> SGVDDDMACHKIPVEADFLYAYS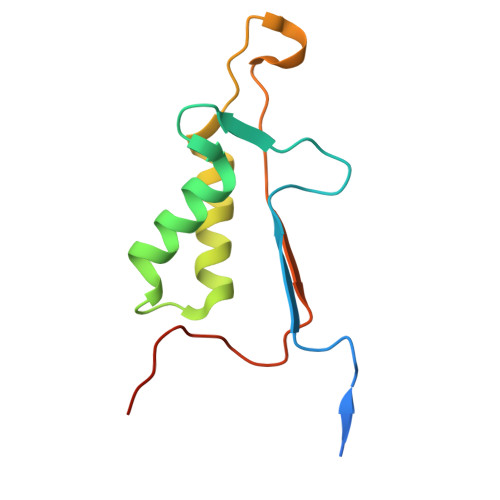TAPGYYSWRNSKDGSWFIQSLCAMLKQYADKLEFMHILTRVNRKVATEFESFSFDATFHAKKQIPCIVSMLTKELYFYHHHHHHH> DDFPPEEDDL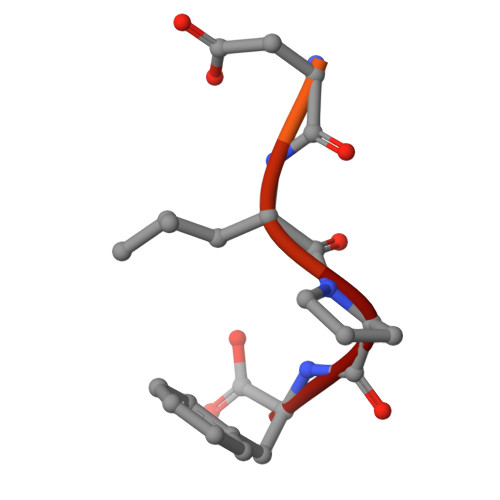PF> GMASLPKRIIKETEKLVSDPVPGITAEPHDDNLRYFQVTIEGPEQSPYEDGIFELELYLPDDYPMEAPKVRFLTKIYHPNIDRLGRICLDVLKTNWSPALQIRTVLLSIQALLASPNPNDPLANDVAEDWIKNEQGAKAKAREWTKLYAKKKP;> AVLGKEAMLKMQTSNVLILGLKGLGVEIAKNVVLAGVKSMTVFDPEPVQLADLSTQFFLTEKDIGQKRGDVTRAKLAELNAYVPVNVLDSLDDVTQLSQFQVVVATDTVSLEDKVKINEFCHSSGIRFISSETRGLFGNTFVDLGDEFTVLDPTGEEPRTGMVSDIEPDGTVTMLDDNRHGLEDGNFVRFSEVEGLDKLNDGTLFKVEVLGPFAFRIGSVKEYGEYKKGGIFTEVKVPRKISFKSLKQQLSNPEFVFSDFAKF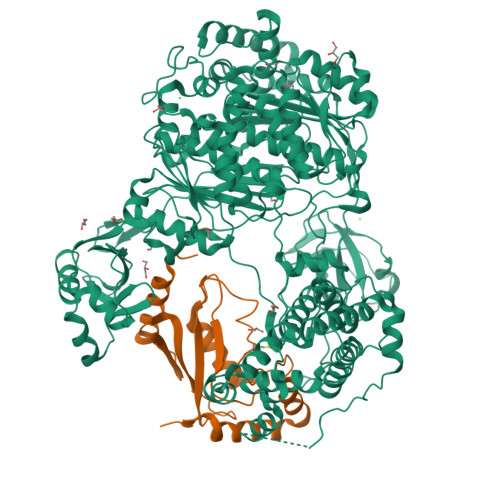DRAAQLHLGFQALHQFAVRHNGELPRTMNDEDANELIKLVTDLSVQQPEVLGEGVDVNEDLIKELSYQARGDIPGVVAFFGGLVAQEVLKACSGKFTPLKQFMYFDSLESLPDPKNFPRNEKTTQPVNSRYDNQIAVFGLDFQKKIANSKVFLVGSGAIGCEMLKNWALLGLGSGSDGYIVVTDNDSIEKSNANRQFLFRPKDVGKNKSEVAAEAVCAMNPDLKGKINAKIDKVGPETEEIFNDSFWESLDFVTNALDNVDARTYVDRRCVFYRKPLLESGTLGTKGNTQVIIPRLTESYSSSRDPPEKSIPLCTLRSFPNKIDHTIAWAKSLFQGYFTDSAENVNMYLTQPNFVEQTLKQSGDVKGVLESISDSLSSKPHNFEDCIKWARLEFEKKFNHDIKQLLFNFPKDAKTSNGEPFWSGAKRAPTPLEFDIYNNDHFHFVVAGASLRAYNYGIKSDDSNSKPNVDEYKSVIDHMIIPEFTPNANLKIQVNDDDPDPNANAANGSDEIDQLVSSLPDPSTLAGFKLEPVDFEKDDDTNHHIEFITACSNCRAQNYFIETADRQKTKFIAGRIIPAIATTTSLVTGLVNLELYKLIDNKTDIEQYKNGFVNLALPFFGFSEPIASPKGEYNNKKYDKIWDRFDIKGDIKLSDLIEHFEKDEGLEITMLSYGVSLLYASFFPPKKLKERLNLPITQLVKLVTKKDIPAHVSTMILEICADDKEGEDVEVPFITIHL> TASTEM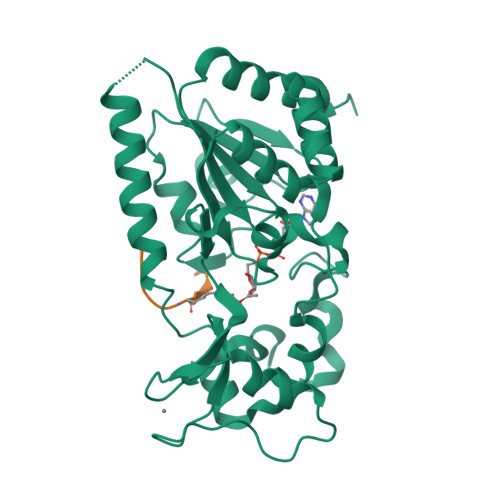SVRKIAAHMKSNPNAKVIFMVGAGISTSCGIPDFRSPGTGLYHNLARLKLPYPEAVFDVDFFQSDPLPFYTLAKELYPGNFRPSKFHYLLKLFQDKDVLKRVYTQNIDTLERQAGVKDDLIIEAHGSFAHCHCIGCGKVYPPQVFKSKLAEHPIKDFVKCDVCGELVKPAIVFFGEDLPDSFSETWLNDSEWLREKITTSGKHPQQPLVIVVGTSLAVYPFASLPEEIPRKVKRVLCNLETVGDFKANKRPTDLIVHQYSDEFAEQLVEELGWQEDFEKILTA;> KGGAKRHRKI> ALWQFNGMIKCKIPSSEPLLDFNNYGCYCGLGGSGTPVDDLDRCCQTHDNCYK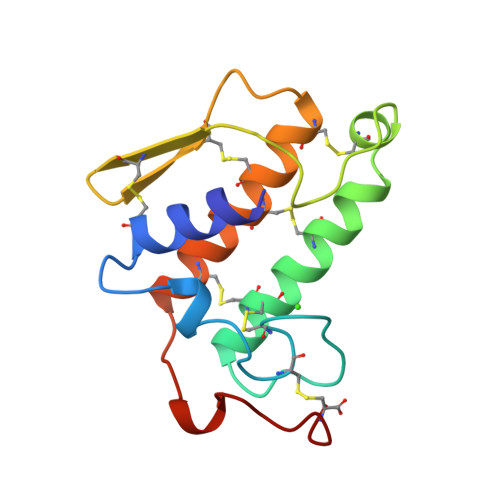QAKKLDSCKVLVDNPYTNNYSYSCSNNEITCSSENNACEAFICNCARNAAICFSKVPYNKEHKNLDKKNC>SKNRISWVGDAVKTDGKKSYYKKVCIDSETLEVGDCVSVIPDDSSKPLYLARVTALWEDSSNGQMFHAHWFCAGTDTVLGATSDPLELFLVDECEDMQLSYIHSKVQVIYKAPSGAGSATYFYQLWYDQDYARFESPPKTQPTEDNKYKFCASCARLA[4x];>GAKRHRKVLRDNY[4x]

In mammals, DNA methylation is stably propagated by DNA methyltransferase 1 (DNMT1) during mitotic division. DNMT1 contains a C-terminal methyltransferase (MTase) domain, preceded by several regulatory domains including a replication-foci-targeting sequence (RFTS), a CXXC zinc finger domain and a pair of bromo-adjacent homology (BAH) domains. Here, we report that DNA methyltransferase 1 (DNMT1) specifically ‘recognizes’ H4K20me3 via its first bromo-adjacent-homology domain (DNMT1BAH1). Here, we show that DNMT1 directly recognizes H4K20me3 through the regulatory domain BAH1, which in turn mediates the chromatin association and enzymatic activation of DNMT1.

To understand the structural basis for the DNMT1BAH1–H4K20me3 interaction, we determined the crystal structure of the BAH1 domain of bovine DNMT1 (bDNMT1BAH1), which shares ~94% sequence identity with hDNMT1BAH1, in complex with the H414–25K20me3 peptide at 2.65 Å resolution. The structure of bDNMT1BAH1 reveals a twisted β-barrel resembling hDNMT1BAH1. The H414–25K20me3 peptide extends along one end of the β-barrel, with the side chain of H4K20me3 inserted into a pocket formed by Y772, W793, D799, and E816 of bDNMT1BAH1 (boxed). Flanking the H414–25K20me3 peptide, the side chains of bDNMT1BAH1 D765 and E818 each form a bidentate hydrogen bond with the backbone amides of H4, and the backbone of bDNMT1BAH1 D765 is further hydrogen bonded to the side chain of H4 R23. Distinct from the typical Kme3 readout that depends on aromatic or other hydrophobic residues only, the BAH1 domain recognizes H4K20me3 via a pocket formed by mixed aromatic and acidic residues. Sequence alignment of the DNMT1 BAH1 domain across different species revealed that the H4K20me2/3-binding sites fall into the most conserved regions. Mutation of hDNMT1BAH1 at or near the corresponding H4K20me3-binding pocket residues (D768A, Y775A, E819A, and E821A) significantly reduced its binding affinity for the H414–25K20me3 or H414–25K20me2 peptide, while introduction of a W796A mutation largely abolishes the hDNMT1BAH1–H414–25K20me3 or hDNMT1BAH1–H414–25K20me2 binding. Strikingly, the H4K20me3 binding by DNMT1BAH1 causes displacement of the autoinhibitory linker, which frees DNMT1 from the linker-mediated autoinhibition and leads to allosteric stimulation of DNMT1, reminiscent of what was previously observed for the DNMT1RFTS–H3K9me3Ub interaction. In the DNA-free state of DNMT1, the H4K20me3-binding site is occluded by the C-terminal portion of the autoinhibitory linker, which likely reinforces the intramolecular RFTS-linker-MTase association, resulting in a direct link between the H4K20me3 binding and enzymatic activation of DNMT1.> GAD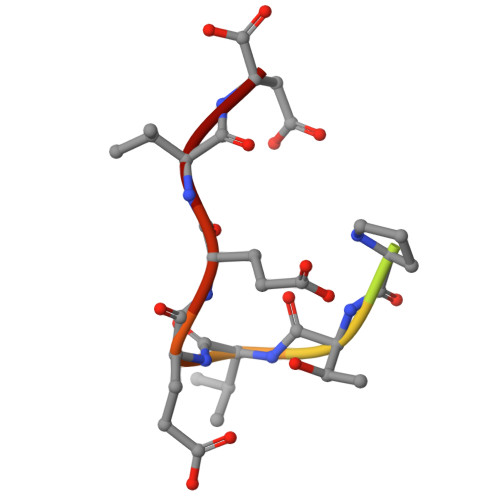NGPTVEEVD> GSHMSPSDLHLPVPGHPIAAIATPVGVGALAIVRISGAGVLDLADRVFRKVHGSGKLAEAAGYTAHFGRLYDGEEMVDEVIALVFRAPRSFTAEQMVEFTCHGGPVVVGRVLRLMLDNGCRLAEPGEFTRRAFLNGRIDLLQAEAIGEMIHARTESAYRTAVSQMKGDLSVRLGGLREQLIRSCALIELELDFSEEDVEFQSRDELTMQIETLRSEVNRLIDSYQHGRIVSEGVSTVIAGKPNAGKSTLLNTLLGQERAIVSHMPGTTRDYIEECFIHDKTMFRLTDTAGLREAGEEIEHEGIRRSRMKMAEADLILYLLDLGTERLDDELTEIRELKAAHPAAKFLTVANKLDRAANADALIRAIADGTGTEVIGISALNGDGIDTLKQHMGDLVKNLDKLHEASVLVTSLRHYEALRNASDALQNALELIAHESETELIAFELRAALDYVGQITGKVVNEEVLNTIFDKFCIGK

MnmE is an evolutionary conserved G protein found in bacteria, fungi, and humans, which together with the protein GidA catalyzes the formation of a carboxymethylaminomethyl-group (cmnm) at the 5 position of the wobble uridine (U34) of tRNAs reading 2-fold degenerated codons ending with A or G, i.e., tRNAArg(UCU), tRNAGln(UUG), tRNAGlu(UUC), tRNALeu(UAA), and tRNALys(UUU). The crystal structure of MnmE from Thermotoga maritima reveals a three-domain protein consisting of an N-terminal tetrahydrofolate-binding domain, a central helical domain, and a canonical Ras-like G domain inserted into the helical domain. On the basis of the common feature that the G domain cycle is regulated by homodimerization, MnmE has been categorized as G protein activated by nucleotide-dependent dimerization (GAD), together with the signal recognition particle (SRP) and its receptor (SR), the regulator of Ni insertion into hydrogenases HypB, the dynamins, the human guanylate binding protein hGBP1, the chloroplast import receptors Toc33/34, the septins, and the Roc-COR tandem found to be mutated in Parkinson disease. The X-ray structures show MnmE to be a constitutive homodimer where the highly mobile G domains face each other in various orientations but are not in close contact as suggested by the GDP-AlFx structure of the isolated domains.

In the case of CtMnmE, a polyethylene glycol (PEG) 6000/NaCl-condition produced diffraction quality crystals in the presence of GPD and GDP-AlFx. CtMnmE·GDP and NoMnmE·GDP (grown in presence of AlFx) crystallized in the space groups I4(1)22 and P4(3)2(1)2, respectively, each with one full length protomer in the asymmetric unit. In both cases homodimers are formed via crystallographic symmetry by means of the N-terminal domains. CtMnmE·GDP crystals were incubated with a 5-F-THF-containing cryoprotectant prior to data collection and in the crystal structure 5-F-THF is found in identical positions as in the NoMnmE·GDP-dimer and in the TmMnmE-dimer. In CtMnmE·GDP however, no Mg2+ is coordinated to the phosphates, and switch I-contacts to GDP are absent. In NoMnmE·GDP a Zn2+-ion tightly links the G domain to symmetry mates, while in CtMnmE·GDP the G domains fix each other by a toothing upside-down arrangement. The corresponding Cβ-Cβ distance in CtMnmE·GDP dimer is somewhat shorter (57 Å), which is due to the different orientation of G domains in this structure and to the different tilting of Gα6. Although both GDP-bound structures have been obtained using GDP and AlFx in the crystallization trials, no electron density for AlFx could be observed.> MQERRALRLGVNGLPNSLEPVNAISNVGPRIVNQIFDTLIARDFFAKGAPGNAIDLVPALAESWERIDEKS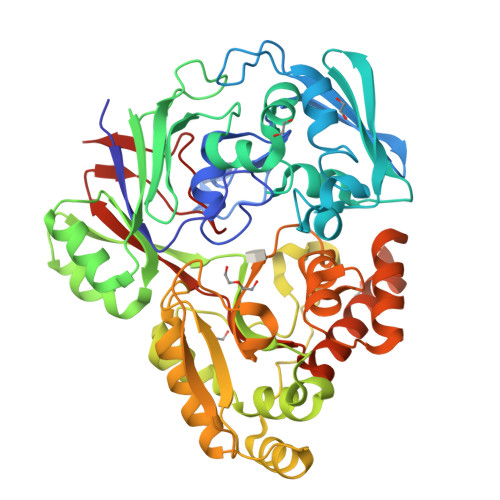VRFKLRQKVMFHDGVELTADDVAYTFSSERLWGPEAIKKIPLGKSYSLDFDEPVVEDKYTVTLRTKTPSYLIETFVASWMSRIVPKEYYKKLGAVDFGNKPVGTGPYKFVEFVAGDRVVLEANDAYWGPKPTASKITYQIVAEPATRVAGLISGEYDIITTLTPDDIQLINSYPDLETRGTLIENFHMFTFNMNQEVFKDKKLRRALALAVNRPIMVEALWKKQASIPAGFNFPNYGETFDPKRKAMEYNVEEAKRLVKESGYDGTPITYHTMGNYYANAMPALMMMIEMWKQIGVNVVMKTYAPGSFPPDNQTWMRNWSNGQWMTDAYATIVPEFGPNGQVQKRWGWKAPAEFNELCQKVTVLPNGKERFDAYNRMRDIFEEEAPAVILYQPYDVYAARKDVHWKPVSFEMMEFRNNLSFGHHHHHH> SDRAMMNAFKEITTMADRINLPRNIVDRTNNLFKQVYEQKSLKGRANDAIASACLYIACRQEGVPRTFKEICAVSRISKKEIGRCFKLILKALETSVDLITTGDFMSRFCSNLCLPKQVQMAATHIARKAVELDLVPGRSPISVAAAAIYMASQASAEKRTQKEIGDIAGVADVTIRQSYR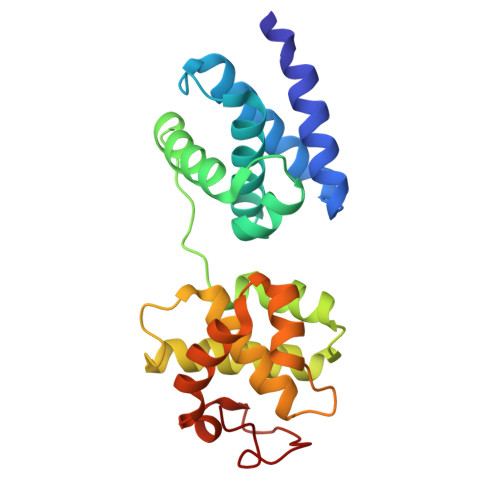LIYPRAPDLFPTDFKFDTPVDKLPQL>[3x]MATHKPINILEAFAAAP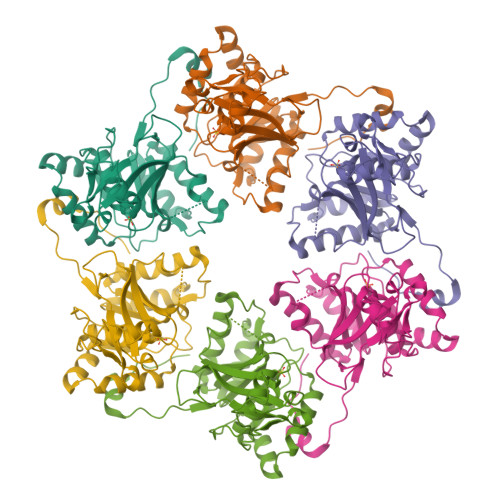PPLDYVLPNMVAGTVGALVSPGGAGKSMLALQLAAQIAGGPDLLEVGELPTGPVIYLPAEDPPTAIHHRLHALGAHLSAEERQAVADGLLIQPLIGSLPNIMAPEWFDGLKRAAEGRRLMVLDTLRRFHIEEENASGPMAQVIGRMEAIAADTGCSIVFLHHASKGAAMMGAGDQQQASRGSSVLVDNIRWQSYLSSMTSAEAEEWGVDDDQRRFFVRFGVSKANYGAPFADRWFRRHDGGVLKPAVLERQRKSKGVPRGEA> MAHHHHHHMNPPSLTAQPGTPVQVMGVVNVTQDSFSDGGKFIDTDRAVEHGLALVAAGAQIIDVGGESTRPGATRIDPGVEAARVTPV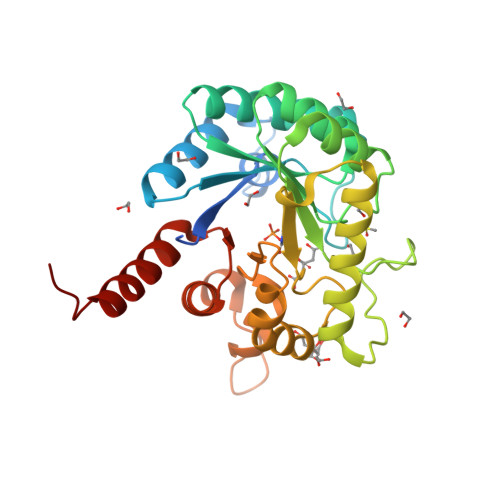IRELAAQGITISIDTMHADVARAALEAGAHIVNDVSGGRADPGMAGVLAEAKVPWILMHWRSVDADHPHRVPGYRDVVAEVRTELLAAVDAAVTAGVEPERLVIDPGLGFAKTAEHNWALLHALPDLVATGVPVLVGASRKRFLGTLLAAADGTPRPPDGRETATAVISVLAAMHGAWGVRVHDVQASVDALKVLGAWTSGEQIG>MMSREADHTIKGFLYQFNKTLNSILSSTDQDEIQIEGIIEDIDIKNSNITNAIQCKYHESKVRHNLSDIYKPILQMLLHFLENDSLNIKYALYAYFPNEQVGVKEVTKSQIEEILSSSNFDYISKYISKIKPPKEQIIKELLGKTSKTTEDKTRIKKYYETSKLETIVDIDKFLRDHFVFEIGLSYEELMNETKNLLMKEGFSLEDVKDLFYPNSIQYIAELSILPEAEKRISSKNKLIDYLKGNKKTAMSRWTSEVLTRKQLLKVRKNQLVPSLNINSRSRYFIIDPDTIDNFDDEFILFVKDYLDKYNSKIKLHTETPCFILKTDVNNLSEYHKRFVSRNIQIITGYIGDTFYFKEFNKEPKRIIKDNWVEFKARISCNSDEVIKCINYKKCDDLYIVGGVDV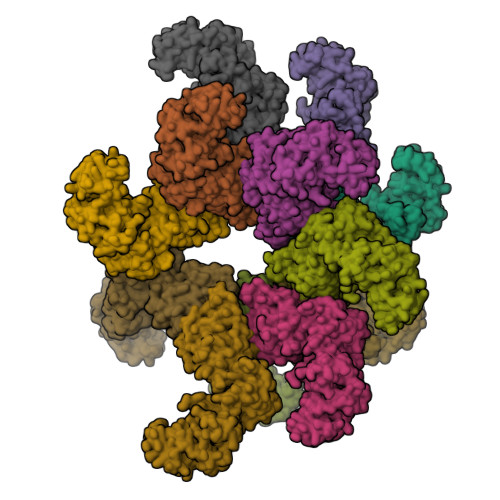SLLDTADVNIENLEINNFRELKYLLSMLKEI[12x]>AHMQHSKSSVHAELRELPESTANLIENSHADDVFSPNMVERLWVLAKSTRDSAQMSDSIISSLSDVLVLSPLEVLASWYAADLLDALLMESLSRKVEISEIE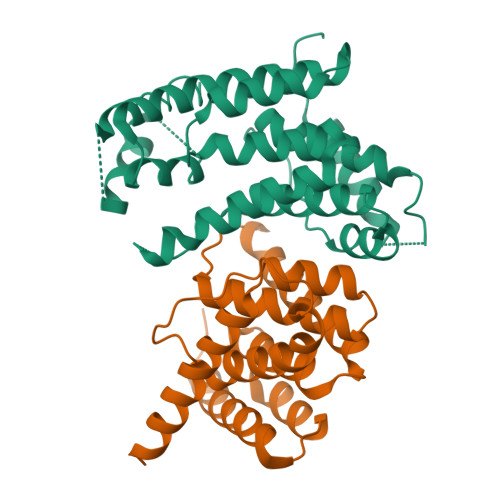EIISLCPKNSSIIRHALLAKLVLFPENTADSLNEVLAAYKNTLDLCSQDKRKQSSVLKINLSKLFTLHSCLSLALQRLGYGDVSKRMYQEIFVPDSDADITPLSFIISWTALNTFAPICTSPKENDVVEKMAMYVRTAIGTLKIQDLKLS[2x]>SKFITSSASDFSDPVYKEIAITNGCINRMSKEELRAKLSEFKLETRGVKDVLKKRLKNYYKKQKLMLKESNFADSYYDYICIIDFEATCEEGNPPEFVHEIIEFPVVLLNTHTLEIEDTFQQYVRPEINTQLSDF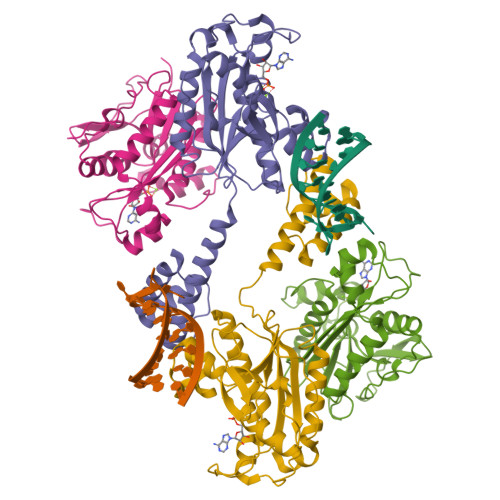CISLTGITQDQVDRADTFPQVLKKVIDLMKLKELGTKYKYSLLTDGSWDMSKFLNIQCQLSRLKYPPFAKKWINIRKSYGNFYKVPRSQTKLTIMLEKLGMDYDGRPNCGLDDSKNIARIAVRMLQDGCELRINEKMHAGQLMSVSSSLPIEGTPPPQMPHFRK[4x]> MVPISPIETVPVKLKPGMDGPKVKQWPLTEEKIKALVEICTEMEKEGKISKIGPENPYNTPVFAIKKKDSTKWRKLVDFRELNKRTQDFWEVQLGIPHPAGLKKKKSATVLDVGDAYFSVPLDEDFRKYTAFTIPSINNETPGIRYQYNVLPQGWKGSPAIFQSSMTKILEPFAAQNPDIVIYQYMDDLYVGSDLEIGQHRTKIEELRQHLLRWGLTTPDKKHQKEPPLLWMGYELHPDKWTVQPIVLPEKDSWTVNDIQKLVGKLNWASQIYPGIKVRQLSKLLRGTKALTEVIPLTEEAELELAENREILKEPVHGVYYDPSKDLIAEIQKQGQGQWTYQIYQEPFKNLKTGKYARMRGAHTNDVKQLTEAVQKITTESIVIWGKTPKFKLPIQKETWETWWTEYWQATWIPEWEFVNTPPLVKLWYQLEKEPIVGAETFYVDGAANR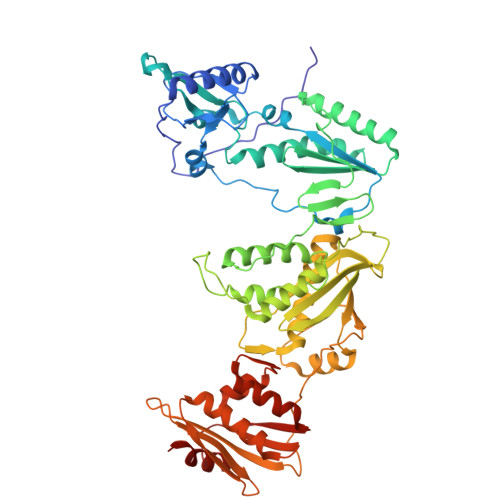ETKLGKAGYVTNKGRQKVVPLTNTTNQKTELQAIYLALQDSGLEVNIVTDSQYALGIIQAQPDKSESELVNQIIEQLIKKEKVYLAWVPAHKGIGGNEQVDKLVSAG>[6x]SNAMGKVLVIYDTRTGNTKKMAELVAEGARSLEGTEVRLKHVDEATKEDVLWADGLAVGSPTNMGLVSWKMKRFFDDVLGDLWGEIDGKIACAFSSSGGWGGGNE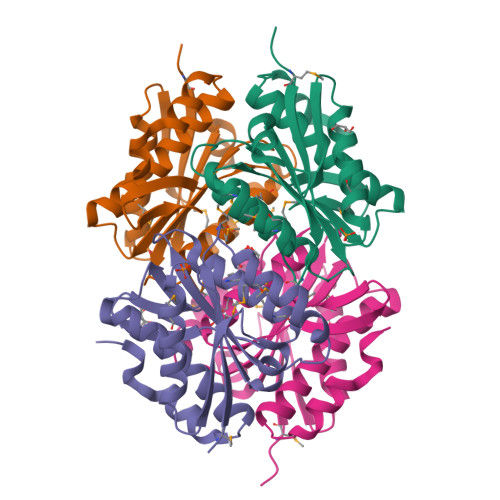VACMSILTMLMNFGFLVFGVTDYVGKKFTLHYGAVVAGEPRSEEEKEACRRLGRRLAEWVAIFVDGRKELLEKIRKDPARFVD> IESD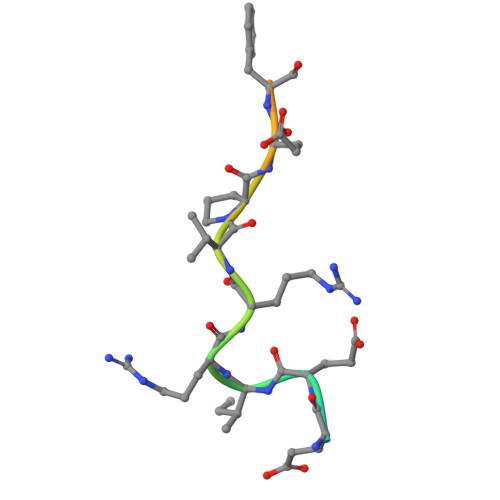EEIRRVPEFGGEAVG> MVVSLRRFHSYANSSRGGATTCLITGGGKGHFALTVSTRGRFYRPLVDDGINLWRRRMGRIHKGWRTWEYQHTRPDPRPFPDPPVNDYFGRSRIWNPIACKLGYVRKKADEWGWPNKPPPPTGLRHSQEFFPFFFERYFPDAEVRLLLDSVLNNETKRPVFQIPCSMSKVELVNYLKNIYGIDNVVRVEVRNRRGRRY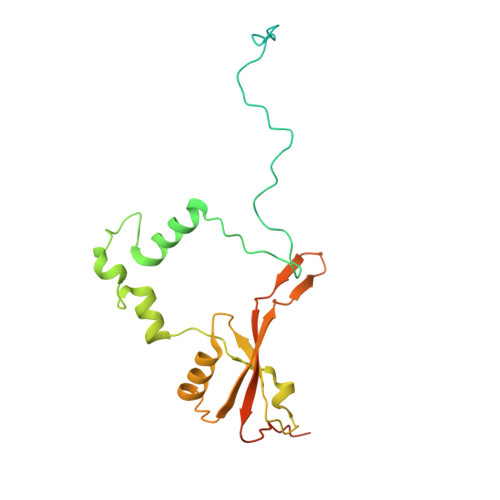KNEVGEIKMMDDYKVAVVELDTPVSVELKQIKGTEDTSDNRPQERITQ>MAVPMDTISGPWGNNGGNFWSFRPVNKINQIVISYGGGGNNPIALTFSSTKADGSKDTITVGGGGPDSITGTEMVNIGTDEYLTGISGTFGIYLDNNVLRSITFTTNLKAHGPYGQKVGTPFSSANVVGNEIVGFLGRSGYYVDAIGTYN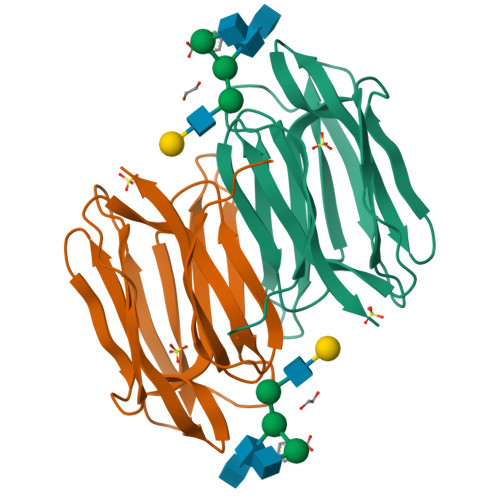RHK[2x]>MSAIENFDAHTPMMQQYLRLKAQHPEILLFYRMGDFYELFYDDAKRASQLLDISLTKRGASAGEPIPMAGIPYHAVENYLAKLVNQGESVAICEQIGDPATSKGPVERKVVRIVTPGTISDEALLQERQDNLLAAIWQDSKGFGYATLDISSGRFRLSEPADRETMAAELQRTNPAELLYAEDFAEMSLIEGRRGLRRRPLWEFEIDTARQQLNLQFGTRDLVGFGVENAPRGLCAAGCLLQYAKDTQRTTLPHIRSITMEREQDSIIMDAATRRNLEITQNLAGGAENTLASVLDCTVTPMGSRMLKRWLHMPVRDTRVLLERQQTIGALQDFTAGLQPVLRQVGDLERILARLALRTARPRDLARMRHAFQQLPELRAQLETVDSAPVQALREKMGEFAELRDLLERAIIDTPPVLVRDGGVIASGYNEELDEWRALADGATDYLERLEVRERERTGLDTLKVGFNAVHGYYIQISRGQSHLAPINYMRRQTLKNAERYIIPELKEYEDKVLTSKGKALALEKQLYEELFDLLLPHLEALQQSASALAELDVLVNLAERAYTLNYTCPTFIDKPGIRITEGRHPVVEQVLNEPFIANPLNLSPQRRMLIITGPNMGGKSTYMRQTALIALMAYIGSYVPAQKVEIGPIDRIFTRVGAADDLASGRSTFMVEMTETANILHNATEYSLVLMDEIGRGTSTYDGLSLAWACAENLANKIKALTLFATHYFELTQLPEKMEGVANVHLDALEHGDTIAFMHSVQDGAASKSYGLAVAALAGVPKEVIKRARQKLRELESIS[2x];>[2x]PNAAATQVDGTQMSLLSVPEETSPAVEALENLDPRSLTPRQALEWIYRLKS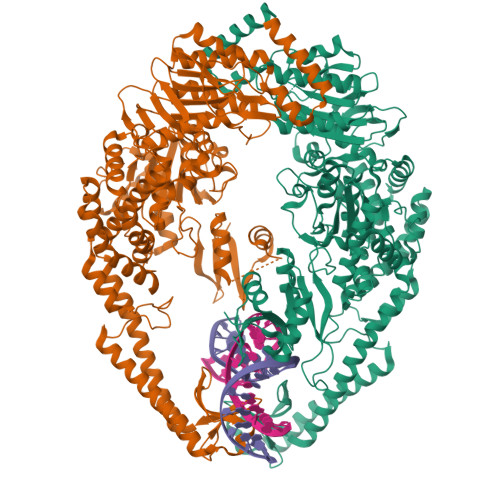LV>GHMPEYDYLFKLLLIGDSGVGKSCLLLRFADDTYTESYISTIGVDFKIRTIELDGKTIKLQIWDTAGQERFRTITSSYYRGAHGIIVVYDVTDQESYANVKQWLQEIDRYASENVNKLLVGNKSDLTTKKVVDNTTAKEFADSLGIPFLETSAKNATNVEQAFMTMAAEIKKRMGLEVLFQ[4x];>[4x]EELYQSILELKPLTLLMTSSTSFSETINQWADILKTTDMEKFSFDSNPINLLELVKQFNLYVDELAITCEANNVWAKERIDSTPNLFALYDNSGGEAIHGHAFVPYYKESIVLRRLFTVDPNTFNLSRFAAFEGPCQLYCAAHADSAWVKIQTLLTL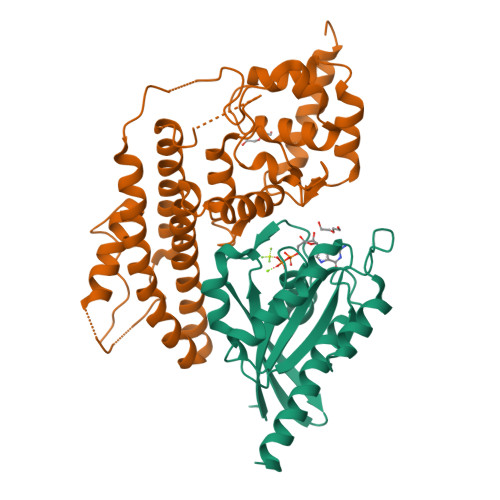GNGIINTLKIIKQAQAFGIDEAVTENLKALKEQFIAFQLAEADIKESLKAPSFAEPLPNKESEFFYPIDEKALAKMNGYQLATICLEELNSPKPSPLIERILSNKKFWKRINSAFESGVFKGRTDDPAGKIAKIREWHQLLQISG> MIFVNDVYKNFGSLEVLKGVTLKVNKGEVVVIIGPSGSGKSTLLRCINLLEEPTKGEVFIDGVKINNGKVNINKVRQKVGMVFQHFNLFPHLTAIENITL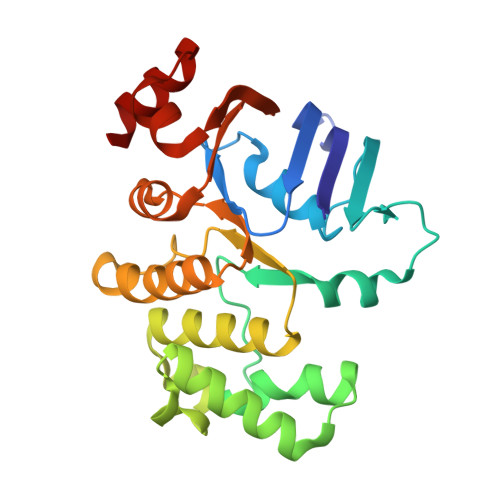APVKVKKMNKKEAEELAVDLLAKVGLLDKKDQYPIKLSGGQKQRLAIARALAMQPEVMLFDEPTSALDPEMVKEVLNVMKQLANEGMTMVVVTHEMGFAREVGDRVIFMDDGVIVEEGTPEEIFYRAKNERTREFLSKIL> DRLTQ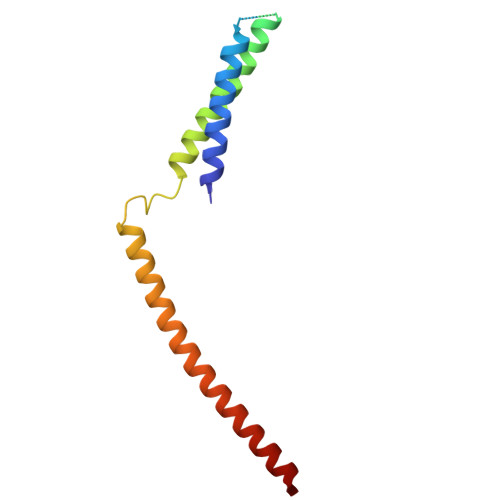LQDAVNSLADQFCNAIGVLQQCGPPASFSNIQTAINKDQPANPTEEYAQLFAALIARTAKDIDVLIDSLPSEESTAALQAASLYKLEEENHEAATCLEDVVYRGDMLLEKIQSALADIAQS Here, we present the structure of an outer-membrane core complex from the iconic F-T4SS encoded by the E. coli pED208 plasmid solved by single-particle cryo-electron microscopy at 3.3 Å resolution. This 2.1 MDa structure, provides an atomic model of the TraB, TraK and TraV proteins and unveils unique stoichiometry relationships between the three proteins. Surprisingly, the complex is formed by two highly flexible concentric rings made by a total of 69 proteins chains arranged in two distinct symmetries. The components that make up this complex include the proteins TraB, TraK and TraV which are homologous to VirB10, VirB9 and VirB7 respectively and are observed throughout the multi-functional T4SS spectrum.

For the outer ring, thirteen ASUOR heteropentamers made of TraK1, TraK2, TraV1CTD, TraV2CTD and TraBCTD(177-186) (labelled −6 to +6 in the clockwise direction) assemble to form the complete OMCCOR. Unexpectedly, the ASUOR segment of the map revealed densities to build and refine more than one molecule of TraK and TraV. Indeed, densities to fit two NTD and CTD domains of TraK (TraK1 and TraK2) were identified. Similarly, densities corresponding to two TraVCTD (TraV1CTD and TraV2CTD) were also observed in the ASUOR segment. The TraKNTD is made up of nine β strands (β1 – β9) in two sheets making a β sandwich domain arrangement. Two such domains from the respective TraK chains (TraK1 and TraK2) are present in a front-to-back arrangement and extensive salt bridge, hydrogen bond and hydrophobic interactions stabilise their interaction. The TraKCTD is made of two α helices (α1 and α2) and six β strands (β10 – β15). The two TraK CTDs are arranged with TraK1 on top of TraK2 and are related by a P2 symmetry. These two TraK CTDs are held together by two anti-parallel TraV chains that wraps the stem of the TraK linkers (α1 – TraK2 and α2 – TraK1). TraV has four β strands per chain making two continuous β-sheets with TraV1 and TraV2 that stabilise the entire OMCCOR complex. TraB also extends into the outer ring with a short stretch of sequence (residues 177–186) at the N-terminal end of the CTD.

>MKKITLLLAGSALLLSGCAGVKSSFDCDATTSDTCMTMTKANQLARDKAAKQAGKPAAGGLPSLVNLPATSAVEVPSASRSAVTPPSGTRTVSTTPPVSAGTSAGVNTNTTTSTLTPRPVAGTPVTTTPSSVAYRPVVSVVTPTPSCQNVRCDNPGTVHPQRSRDQIATVWIAPWVDSDNAFHQPGRVSFVVSPADWVLPARVN[26x];>[13x]PGMMDSQEFS;>[26x]AQSPATISLPQGGQFRLSISNTDPNMIFIPGDKVTAITAPGGMLADKRLTTAGGVLFTSVATRTFTIFVETALGQTFSVVATPVKGEGRVYRLMSAEPPSRPETRKWETAQAYEKLLISLNRAVLTGDIPDGYGEVKPLSDGIRLPGGFSVTPLKAWAGDQLRADRYELRNANTWGVALREQDFWKPGVRAVMFDNNAQTLMGGGRMTVTVIRGNG>FNLPPGNYKKPKLLYCSNGGHFLRILPDGTVDGTRDRSDQHIQLQLSAESVGEVYIKSTETGQYLAMDTDGLLYGSQTPNEECLFLERLEENHYNTYISKKHAEKNWFVGLKKNGSCKRGPRTHYGQKAILFLPLPVSSD[2x];>SNNKRAPYWTNTEKMEKRLHAVPAANTVKFRCPAGGNPMPTMRWLKNGKEFKQEHRIGGYKVRNQHWSLIMESVVPSDKGNYTCVVENEYGSINHTYHLDVVERSPHRPILQAGLPANASTVVGGDVEFVCKVYSDAQPHIQWIKHVEKNGSKYGPDGLPYLKVLKAAGVNTT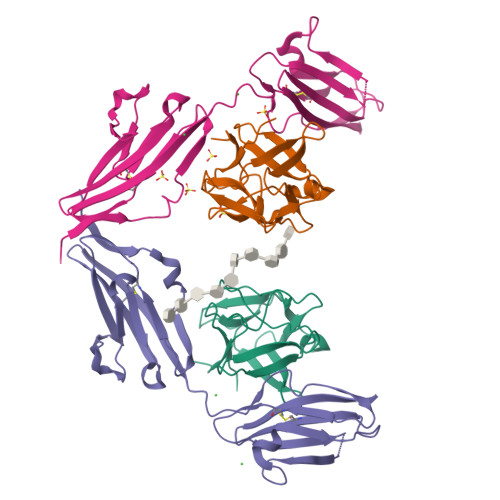DKEIEVLYIRNVTFEDAGEYTCLAGNSIGISFHSAWLTVLPAPGRE[2x]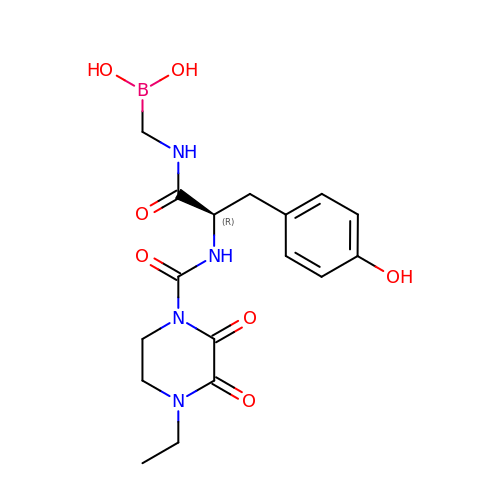N-[(dihydroxyboranyl)methyl]-Nalpha-[(4-ethyl-2,3-dioxopiperazin-1-yl)carbonyl]-D-tyrosinamide | C17 H23 B N4 O7 | INXKLMQPFNYGIK-CYBMUJFWSA-N> MASSINGRKPSEIFKAQALLYKHIYAFIDSMSLKWAVEMNIPNIIQNHGKPISLSNLVSILQVPSSKIGNVRRLMRYLAHNGFFEIITKEEESYALTVASELLVRGSDLCLAPMVECVLDPTLSGSYHELKKWIYEEDLTLFGVTLGSGF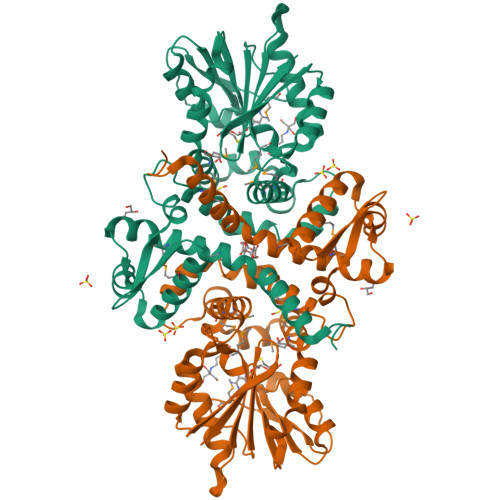WDFLDKNPEYNTSFNDAMASDSKLINLALRDCDFVFDGLESIVDVGGGTGTTAKIICETFPKLKCIVFDRPQVVENLSGSNNLTYVGGDMFTSIPNADAVLLKYILHNWTDKDCLRILKKCKEAVTNDGKRGKVTIIDMVIDKKKDENQVTQIKLLMDVNMACLNGKERNEEEWKKLFIEAGFQHYKISPLTGFLSLIEIYP(4-nitrophenyl) hexanoate | C12 H15 N O4 | 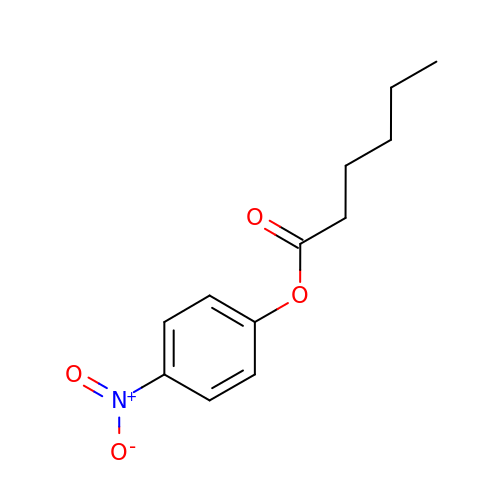OLRXUEYZKCCEKK-UHFFFAOYSA-N> HHHHHMVDAAVAEK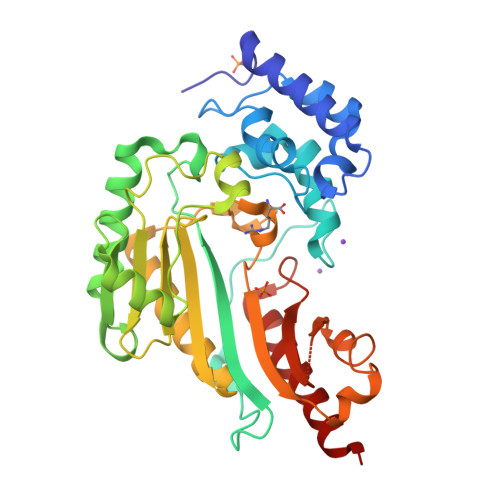LEAGFQKLQEATNCKSLLKKHLTREIFDKIKDLKTSFGSTLLDVIQSGVENLDSGFGVYAPDAEAYSVFNDLFEPMICDYHTGFKPGDAHPPRDFGDLETFGNLDPEGAFIVSTRVRCGRSLAGYAFNPCLTEANYKEMEEKVVASLSSLEGELKGTYYPLTGMTKEVQTQLIQDRFLFKEGDRFLQAANACRYWPTGRGIYHNDAKTFLVWCNEEDHLRIISMQKGGDLKAVYARLVNAINEIEKRIPFSHHDKYGFLTFCPTNLGTTIRASVAIALPKLAADLAKLEEAAGKFNLQVRGTAGEHTEAEGGVYDISNKRRMGLTEYQAVKEMYDGLQELIRMEKEAA> QEGDFPMPFISAKSSPVIPLDGSVKIQCQAIREAYLTQLMIIKNSTYREIGRRLKFWNETDPEFVIDHMDANKAGRYQCQYRIGHYRFRYSDTLELVVTGLYGKPFLSADRGLVLMPGENISLTCSSAHIPFDRFSLAKEGELSLPQHQSGEHPANFSLGPVDLNVSGIYRCYGWY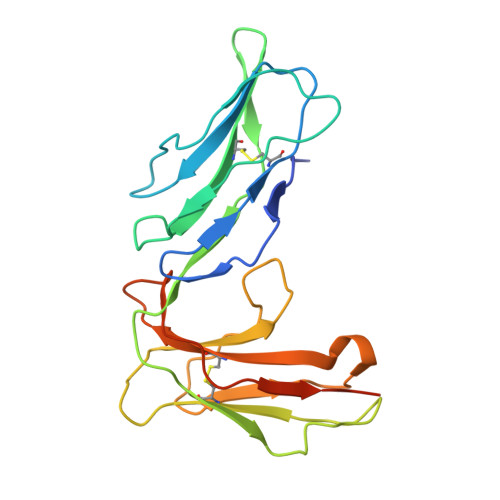NRSPYLWSFPSNALELVVTAIDGRAHHHHHH> MTTLTRQDLNFGQVVADVLCEFLEVAVHLILYVREVYPVGIFQKRKKYNVPVQMSCHPELNQYIQDTLHCVKPLLEKNDVEKVVVVILDKEHRPVEKFVFEITQPPLLSISSDSLLSHVEQLLAAFILKISVCDAVLDHNPPGCTFTVLVHTREAATRNMEKIQVIKDFPWILADEQDVHMHDPRLIPLKTMTSDILKMQLYVEE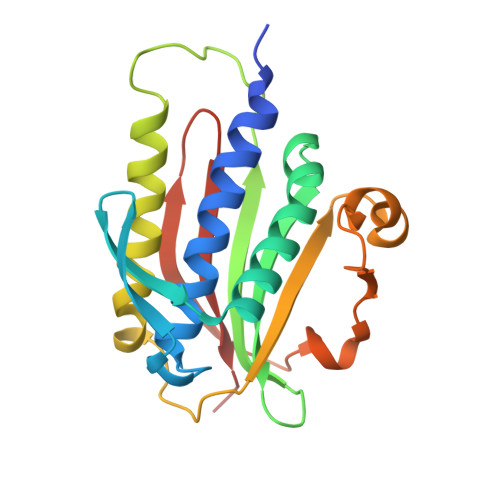RAHKGS(3R,4R)-4-[4-(2-Chlorophenyl)piperazin-1-yl]-1,1-dioxothiolan-3-ol 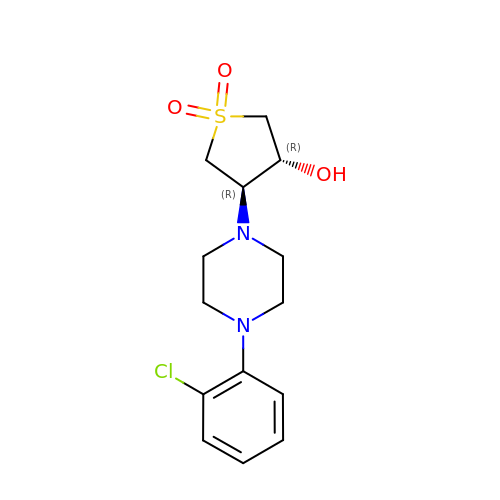| C14 H19 Cl N2 O3 S | CRYVRLLTCKZRFB-KBPBESRZSA-N> MKHTELRAAVLDALEKHDTGATFFDGRPAVFDEADFPAVAVYLTGAEYTGEELDSDTWQAELHI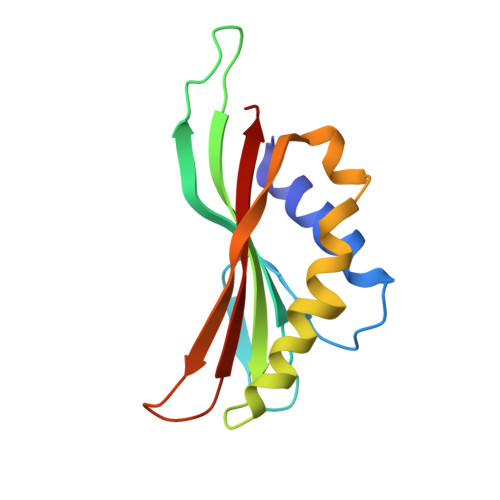EVFLPAQVPDSELDAWMESRIYPVMSDIPALSDLITSMVASGYDYRRDDDAGLWSSADLTYVITYEM> MVEATAQETDRPRFSFSIAAREGKARTGTIEMKRGVIRTPAFMPVGTAATVKALKPETVRATGADIILGNTYHLMLRPGAERIAKLGGLHSFMGWDRPILTDSGGYQVMSLSSLTKQSEEGVTFKSHLDGSRHMLSPERSIEIQHLLGSDIVMAFDECTPYPATPSRAASSMERSMRWAKRSRDAFDSRKEQAENAALFGIQQGSVFEN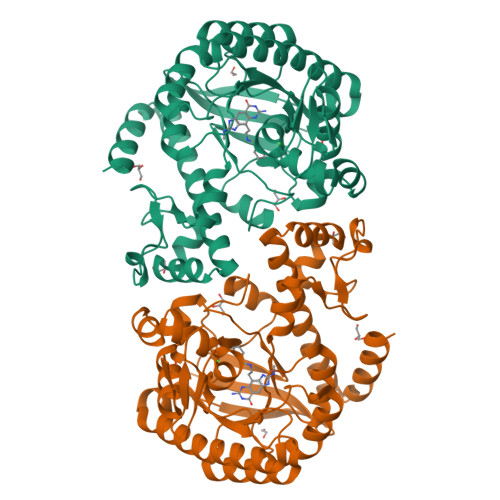LRQQSADALAEIGFDGYAVGGLAVGEGQDEMFRVLDFSVPMLPDDKPHYLMGVGKPDDIVGAVERGIDMFDCVLPTRSGRNGQAFTWDGPINIRNARFSEDLKPLDSECHCAVCQKWSRAYIHHLIRAGEILGAMLMTEHNIAFYQQLMQKIRDSISEGRFSQFAQDFRARYFARN> GGNSFVGLRVVAKWSSNGYFYSGKITRDVGAGKYKLLFDDGYECDVLGKDILLCDPIPLDTEVTALSEDEYFSAGVVKGHRKESGELYYSIEKEGQRKWYKRMAVILSLEQGNRLREQY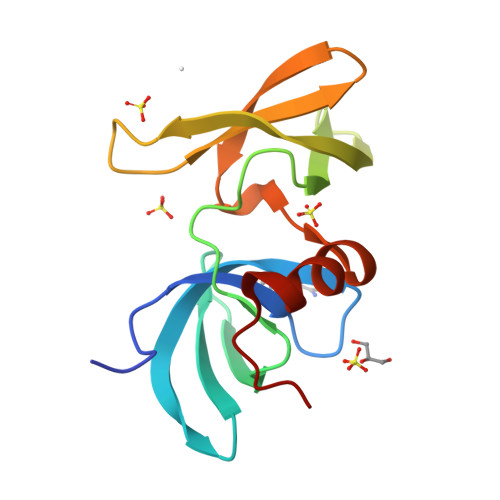GLGPYE RlmCD is a recently identified MTase for ribosomal RNA in S. pneumoniae. Similar to its homologue YefA in B. subtilis, RlmCD can catalyze m5U methylation for both U747 and U1939 of 23S rRNA, whereas these two modifications are catalyzed by two different enzymes RlmC and RumA, respectively, in E. coli. Our structural evidences indicate that RlmCD is a MTase that belongs to the RFM family. All together, our in-vitro experiments confirmed that RlmCD is a 23S rRNA MTase specific for U747.

The RlmCDs construct used for crystallization was designed based on the sequence alignment with its homologue in E.coli, RumA, whose structure has been previously determined. In this structure, each asymmetric unit contains only one protein molecule. The overall structure of RlmCDs highly resembles that of RumA with a RMSD of 1.9Å for the backbone Cα atoms. It is composed of three distinct domains representing the residues 1–63, 128–261, and 281–454, respectively. The N-terminal TRAM domain is the smallest domain formed as a five-stranded antiparallel β-barrel (β1 to β5), which is also known as the typical OB fold. The central domain comprises a six-stranded β-sheet (β6 to β11) stacked against two α-helices (α3 and α4). The C-terminal catalytic domain exhibits a typical SAM-dependent MTase fold in which the β-strands (β14 to β20) of a seven-stranded β-sheet and α-helices (α5 to α10) are connected in an interleaved mode. Most strikingly, compared with those in RumA, the linker regions between α3 and β8 (linker A) and between β10 and β11 (linker B) in the central domain are evidently longer in RlmCD. Careful structural comparison between RlmCDs and RumA revealed the noticeable differences in the lengths of the two linker regions (liner A and B) in the central domains. These two linker regions both have 13 amino acids in RlmCD while their lengths in RumA are 3 and 6 residues, respectively. Given that the overall structures of RumA and RlmCD are highly similar and that they both exhibit MTase activity for U1939 in 23S rRNA, it is quite interesting that RlmCD doesn’t possess an iron-sulfur cluster as RumA, but instead that the corresponding region in RlmCD (residues 72–81) folds as a short α-helix.

> MLKKNDIVEVEIVDLTHEGAGVAKVDGLVFFVENALPSEKILMRVLKVNKKIGFGKVEKYLVQSPHRNQDLDLAYLRSGIADLGHLSYPEQLKFKTKQVKDSLYKIAGIADVEVAETLGMEHPVKYRNKAQVPVRRVNGVLETGFFRKNSHNLMPLEDFFIQDPVIDQVVVALRDLLRRFDLKPYDEKEQSGLIRNLVVRRGHYSGQIMVVLVTTRPKVFRVDQLIEQVIKQFPEIVSVMQNINDQNTNAIFGKEWRTLYGQDYITDQMLGNDFQIAGPAFYQVNTEMAEKLYQTAIDFAELKKDDVIIDAYSGIGTIGLSVAKHVKEVYGVELIPEAVENSQKNASLNKITNAHYVCDTAENAMKKWLKEGIQPTVILVDPPRKGLTESFIKASAQTGADRIAYISCNVATMARDIKLYQELGYELKKVQPVDLFPQTHHVETVALLSKLDVD>MSKLASECVANILNDWYIAIKQQDAESAERYFEEVKPLFDEMEEDQEVLMYYSLLEERHKMLLYQVKGEELPPHSYFNENHAEEIKKTDHMIEYYFFLFEALYESHKRNFEKAITLFKIAEKKLKDIPDCIERAEFYSKVASMYMMLRQSLISLNYINDSIQIYRENEGYKRKLATSLMIVGQNYTDLGLYEKAEESFLEAIRISRVLHDSLFTALIHHNLSITYSAANRSQDCINALKKAIRNKEWRDSVYYINSLYMFLKELYKIGDVNKMPYYYKKTKEYFKRKENKVYEAKINIIYGLLQQDQRKSIETCRGGISYLYEVNDLDSVFDLSLVISEHCEKHGLYKEALEFSKHAILAEEKMRHLEGL[2x];>ERPVGT[2x]

Proteins of the RRNPPA family are the most frequent pheromone receptors in Bacillota and use small secreted oligopeptides as pheromones. While most members of the RRNPPA family act as transcriptional factors through DNA binding, Rap receptors are specialized members that exhibit the capability to develop their function by interaction with specific protein targets. Binding of the pheromone produced from the propeptide, which is named Phr in this RRNPPA subfamily, induces Rap receptor inhibition. Our results reveal that distinct maturation processes generate multiple mature pheromones, which bind to receptors with varying affinities but produce identical structural and biological responses.

The Rap-Phr system from phage phi105 caught our attention as its Phr (Phr105) carried 2 identical copies of the putative mature pheromone (ERPVGT). To comprehend the interaction between Rap105 and its predicted mature pheromone (ERPVGT), an MST analysis was performed revealing an EC50 of 34nM with a Hill coefficient of 1.41. To further understand the recognition by Rap105, we solved the structure of Rap105-ERPVGT (Rap-Phr105) complex at 2.5 Å resolution. Rap-Phr105 complex crystallized in spatial group P21 with 2 Rap molecules per asymmetric forming a dimer with similar organization to the observed in Rap3T and other Raps. The structure of the receptor showed the classical architecture of Rap receptors with N-terminal 3HB domain (residues 1–67) followed by 7 TPRs (residues 89–367). Analysis of the pheromone’s binding pocket unveiled Asn220, corresponding to Asn226 in Rap3T, as the conserved Rap Asn that anchors the pheromone. A further 16 receptor residues (Q65, S142, M145, M146, T176, I180, Q183, D187, L216, I223, Y252, Y258, Y292, K295, D328, and D332) formed direct contacts with the pheromone. Pheromones in both receptors are well anchored by their N- and C-terminal ends and present an Arg in position two whose side chain shows a similar interaction with the receptor, mainly through a salt bridge with an Asp residue located at identical position (D187/D193 and D338/D332 for Rap105 and Rap3T, respectively). However, the pheromone Phr105 shows null or weak interactions through two of its 6 amino acids (Pro3 and Gly5). Also, the presence of this proline in the middle of the pheromone restricts the conformational freedom of the peptide, while in the Phr3T this Pro is a Gly that increases pheromone freedom and mediates interactions with 2 tyrosines (Y151 and Y225) of Rap3T receptor.>MGSMTSDTARSYRFPEGFLWGAATAAYQIEGSSMADGAGESIWDRFSHTPGNMKDGDTGDVACDHYNRWREDIELMKRLNLQAYRFSVSWSRVIPQGRGAINPKGLAFYDRLVDGLLEAGIEPLATLYHWDLPAALDDRGGWLNPDIADWFADYGQVLFEKFKGRVKTWGTINEPWVIVDGGYLHGALAPGHRSAYEAVIAGHNVLRAHGAAVRRFREVGEGQIGIVLNIEPKYPASDKPEDEAARRRAEAQMNRWFLDPLMGRGYPEELTDVYGAAWREFPKEDFELIAEPTDWMGLNWYTRAVPENAPDAWPTRSRPVRQTQHAHTETGWEVYPPALTDTLVWLSEQTGGKLPLMVTENGSAWYDPPHAIDGRIHDPMRVHYLQTHIKALHDAIGKGVDLRGYMAWSLLDNLEWSLGYSKRFGIVHVNFATQERTIKDSGLLYAEVIKTHGDVLNTLKLHHHHHH[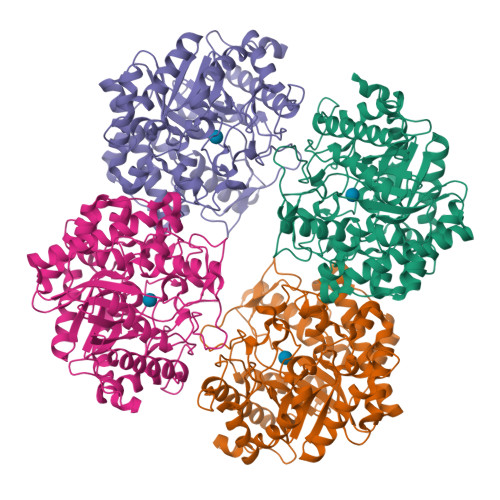4x]>[2x]DRHHHHHHKLVPLAPADRAPAVGQFWHVTDLHLDPTYHITDDRTKVCASSKGANASNPGPFGDVLCDSPYQLILSAFDFIKNSGQEASFMIWTGDSPPHVPVPELSTGTVIKVITNMTMTVQNLFPNLQVFPALGNHDYWPQDQLPIVTSKVYSAVADLWKPWLGEEAISTLKKGGFYSQK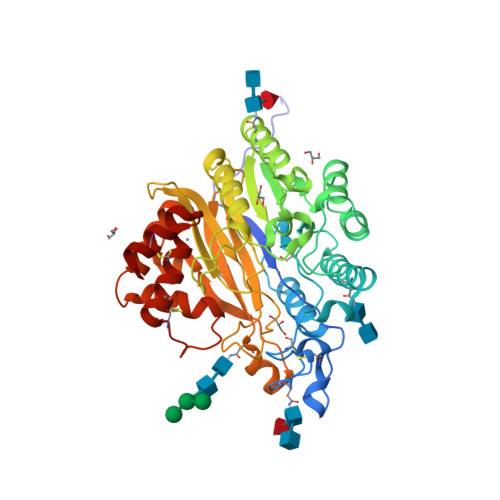VASNPGLRIISLNTNLYYGPNIMTLNKTDPANQFEWLENTLNSSLWNKEKVYIIAHVPVGYLPYATDTPAIRQYYNEKLLDIFRRYSSVIAGQFYGHTHRDSLMVLSDKNGNPLNSVFVAPAVTPVKGVLQKETNNPGVRLFQYKPGDYTLLDMVQYYLNLTEANLKGESNWTLEYVLTQAYSVADLQPKSLYALVQQFATKDSKQFLKYYHYYFVSYDSSATCDQHCKTLQVCAIMNLDSMSYDDCLKQHL2-methyl-~{N}-[(2~{S})-2-methylsulfonylcyclopentyl]pyridin-3-amine | C12 H18 N2 O2 S | 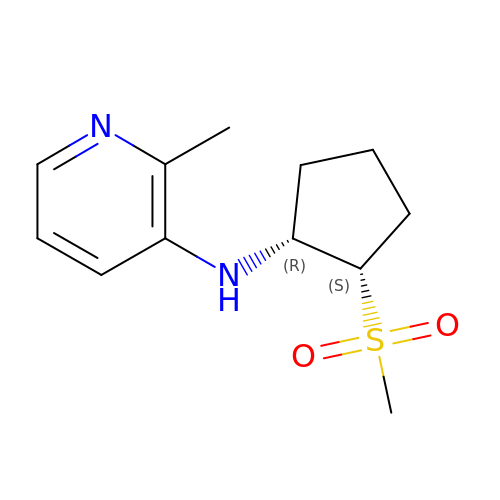BFFKQDIRHHTNOE-NEPJUHHUSA-N2-[(~{E})-2-thiophen-2-ylethenyl]benzoic acid | C13 H10 O2 S | 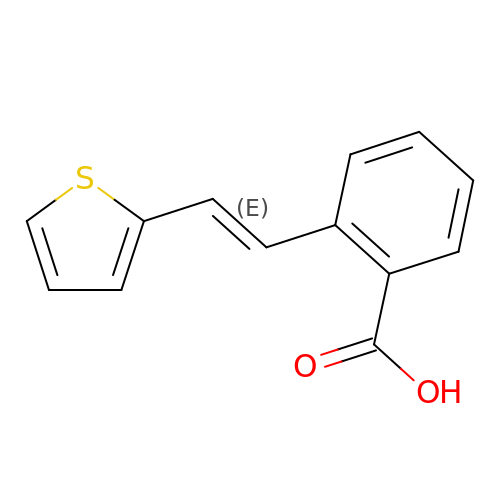ISSJZCAENPGUEW-BQYQJAHWSA-N Cas12a2 is a CRISPR-associated nuclease that performs RNA-guided, sequence-nonspecific degradation of single-stranded RNA, single-stranded DNA and double-stranded DNA following recognition of a complementary RNA target, culminating in abortive infection. However, it was recently discovered that Cas12a2 from Sulfuricurvum sp. PC08-66 instead relies on abortive infection—that is, dormancy or cell death in response to the presence of an invader—to achieve population-level immunity, preventing the replication and transmission of plasmids. Cas12a2 adopts a bilobed architecture, with a recognition (REC) lobe comprising the REC1 and REC2 domains and the nuclease (NUC) lobe consisting of the PI, wedge (WED), RuvC nuclease, ZR and Cas12a2-specific insertion domains. To understand the unique mechanisms of activation, substrate capture and indiscriminate nuclease activity underlying the function of Cas12a2, we carried out biochemical, structural and in vivo analyses, including determining cryo-electron microscopy (cryo-EM) structures of autoinhibited Cas12a2–crRNA (binary complex) associated with an RNA target (ternary complex) and bound to both an RNA target and a dsDNA collateral substrate mimetic (quaternary complex).

To gain insights into the function of Cas12a2, we first purified a binary complex consisting of catalytically active Cas12a2 and a mature crRNA and determined the structure using cryo-EM to a global resolution of 3.2 Å. The quality of the map allowed de novo modelling of most of Cas12a2, aside from the flexible PFS-interacting (PI) and ZR domains. Of note, seven nucleotides of pre-ordered crRNA sit at the interface between REC1 and REC2 in a conformation in which bases are solvent-exposed and primed for target recognition. This region is towards the 3′ end of the crRNA, and the intervening sequence between the 5′ crRNA stem–loop and this pre-ordered guide is disordered in our structure, probably owing to flexibility. Our structure suggests that Cas12a2–crRNA–target strand (TS) duplex formation may initiate and propagate from the 3′ end of the crRNA, enabling Cas12a2 to target phage that have escaped surveillance by Cas12a through mutagenesis of the PAM or 5′ seed regions. Inspection of the RuvC active site in the autoinhibited binary complex reveals that the catalytic triad (D848, E1063 and D1213) is buried within a solvent-excluded pocket. In the binary complex (Cas12a2–crRNA), the active site is occluded. The 3′ end of the crRNA is a pre-ordered seed, and the PI domain is flexible.

> MLHAFTNQYQLSKTLRFGATLKEDEKKCKSHEELKGFVDISYENMKSSATIAESLNENELVKKCERCYSEIVKFHNAWEKIYYRTDQIAVYKDFYRQLSRKARFDAGKQNSQLITLASLCGMYQGAKLSRYITNYWKDNITRQKSFLKDFSQQLHQYTRALEKSDKAHTKPNLINFNKTFMVLANLVNEIVIPLSNGAISFPNISKLEDGEESHLIEFALNDYSQLSELIGELKDAIATNGGYTPFAKVTLNHYTAEQKPHVFKNDIDAKIRELKLIGLVETLKGKSSEQIEEYFSNLDKFSTYNDRNQSVIVRTQCFKYKPIPFLVKHQLAKYISEPNGWDEDAVAKVLDAVGAIRSPAHDYANNQEGFDLNHYPIKVAFDYAWEQLANSLYTTVTFPQEMCEKYLNSIYGCEVSKEPVFKFYADLLYIRKNLAVLEHKNNLPSNQEEFICKINNTFENIVLPYKISQFETYKKDILAWINDGHDHKKYTDAKQQLGFIRGGLKGRIKAEEVSQKDKYGKIKSYYENPYTKLTNEFKQISSTYGKTFAELRDKFKEKNEITKITHFGIIIEDKNRDRYLLASELKHEQINHVSTILNKLDKSSEFITYQVKSLTSKTLIKLIKNHTTKKGAISPYADFHTSKTGFNKNEIEKNWDNYKREQVLVEYVKDCLTDSTMAKNQNWAEFGWNFEKCNSYEDIEHEIDQKSYLLQSDTISKQSIASLVEGGCLLLPIINQDITSKERKDKNQFSKDWNHIFEGSKEFRLHPEFAVSYRTPIEGYPVQKRYGRLQFVCAFNAHIVPQNGEFINLKKQIENFNDEDVQKRNVTEFNKKVNHALSDKEYVVIGIDRGLKQLATLCVLDKRGKILGDFEIYKKEFVRAEKRSESHWEHTQAETRHILDLSNLRVETTIEGKKVLVDQSLTLVKKNRDTPDEEATEENKQKIKLKQLSYIRKLQHKMQTNEQDVLDLINNEPSDEEFKKRIEGLISSFGEGQKYADLPINTMREMISDLQGVIARGNNQTEKNKIIELDAADNLKQGIVANMIGIVNYIFAKYSYKAYISLEDLSRAYGGAKSGYDGRYLPSTSQDEDVDFKEQQNQMLAGLGTYQFFEMQLLKKLQKIQSDNTVLRFVPAFRSADNYRNILRLEETKYKSKPFGVVHFIDPKFTSKKCPVCSKTNVYRDKDDILVCKECGFRSDSQLKERENNIHYIHNGDDNGAYHIALKSVENLIQMK>HMNDMAHPNSAVLADFIPVQLAKPVPQRITLELTAYGFARAHCLSNGITDEEGFVQVYKTVKEKFDKYAVSPAQIKQRQLVYFPKLTDIRFGDGNFDIADPEPDQAHLRLFDIKKDPRGADLKTRHESYAKVVGKGLEQMFEGTLEAPDDLIHVTCSGYLAPSPAERMVADRGWFETTVTHSYNMGCYGAFPAIKMAHGMLASAQWGATPPKTRVDIAHTELMSAHNNIAESRVDNIISATLFSDGLIKYSVYPEDELRRQGLRGLRILAMSEHLLPDSADTMTWVPGSHQFVMTLSPLVPAIIKRHVR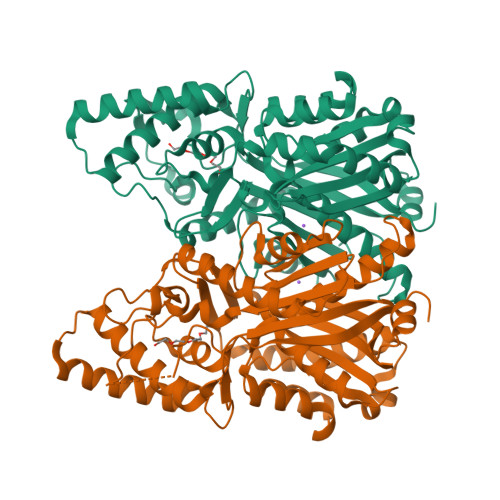AFAVDLLRRAGMDFERDKDALSFAIHPGGPKIVDHVQEELGLAEDQVAISKSVFLENGNMSSSTIPHILKAYLEEATVGTRIACLGFGPGLTAAGLVLEKI[8x]>[60x]MPWWYRRRSYNPWRRRNWFRRPRKTIYRRYRRRRRWVRRKPFYKRKIKRLNIVEWQPKSIRKCRIKGMLCLFQTTEDRLSYNFDMYEESIIPEKLPGGGGFSIKNISLYALYQEHIHAHNIFTHTNTDRPLARYTGCSLKFYQSKDIDYVVTYSTSLPLRSSMGMYNSMQPSIHLMQQNKLIVPSKQTQKRRKPYIKKHISPPTQMKSQWYFQHNIANIPLLMIRTTALTLDNYYIGSRQLSTNVTIHTLNTTYIQNRDWGDRNKTYYCQTLGTQ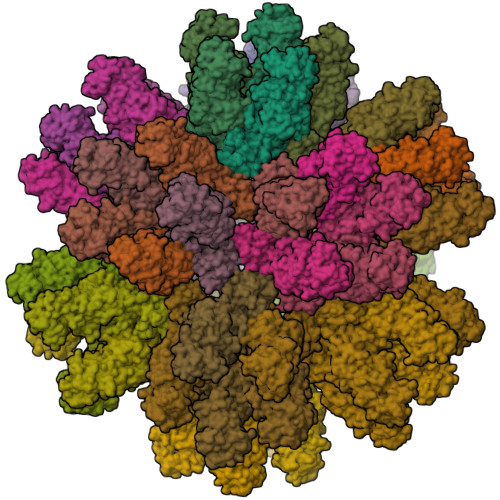RYFLYGTHSTAQNINDIKLQELIPLTNTQDYVQGFDWTEKDKHNITTYKEFLTKGAGNPFHAEWITAQNPVIHTANSPTQIEQIYTASTTTFQNKKLTDLPTPGYIFITPTVSLRYNPYKDLAERNKCYFVRSKINAHGWDPEQHQELINSDLPQWLLLFGYPDYIKRTQNFALVDTNYILVDHCPYTNPEKTPFIPLSTSFIEGRSPYSPSDTHEPDEEDQNRWYPCYQYQQESINSICLSGPGTPKIPKGITAEAKVKYSFNFKWGGDLPPMSTITNPTDQPTYVVPNNFNETTSLQNPTTRPEHFLYSFDERRGQLTEKATKRLLKDWETKETSLLSTEYRFAEPTQTQAPQEDPSSEEEEESNLFERLLRQRTKQLQLKRRIIQTLKDLQKLE>MHEWALADAIVRTVLDYAQREGASRVKAVRVVL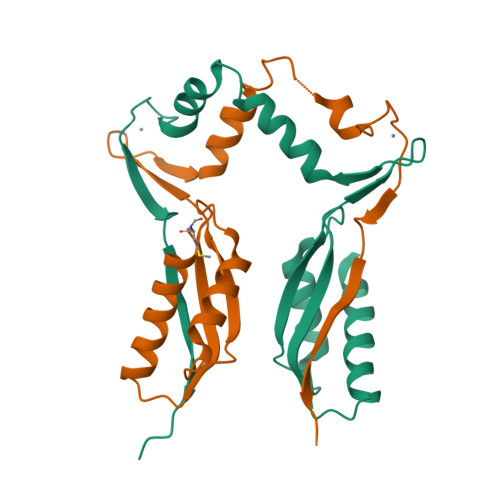GELQDVAEDIVKFAMEQLFAGTIAEGAEIEFVEEEAVFKCRNCNYEWKLKEVKDKFDERIKEDIHFIPEVVHAFLACPKCGSHDFEVVKGRGVYVAGIKIEKEGGS[4x]>[2x]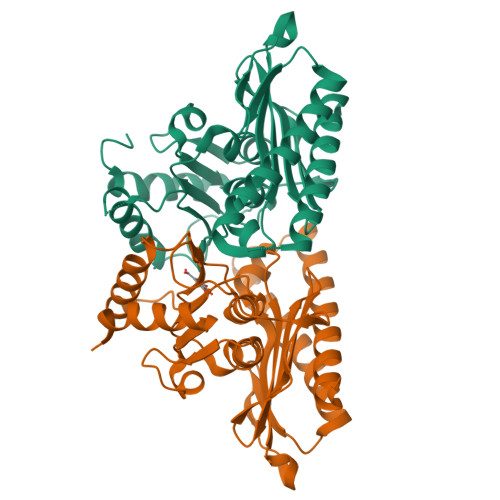MQPMLNIALRAARSAGELIFRSIERLDVISVNEKDAKDYVTEVDRAAEQTIVAALRKAYPTHAIMGEEGGLIEGSGEGADYLWVIDPLDGTTNFIHGVPHFAVSIACKYKGRLEHAVVLDPVRQEEFTASRGRGAALNGRRLRVSGRKSLEGALLGTGFPFRDNQIDNLDNYLNMFRSLVGQTAGIRRAGAASLDLAYVAAGRYDAFWEFGLSEWDMAAGALLVQEAGGLVSDFTGSHEFLEKGHIVAGNTKCFKALLTTIQPHLPPSLKR> FNLPPGNYKKPKLLYCSNGGHFLRILPDGTVDGTRDRSDQHIQLQLSAESVGEVYIKSTETGQYLAMDTDGLLYGSQTPNEECLFLERLEENHYNTYISKKH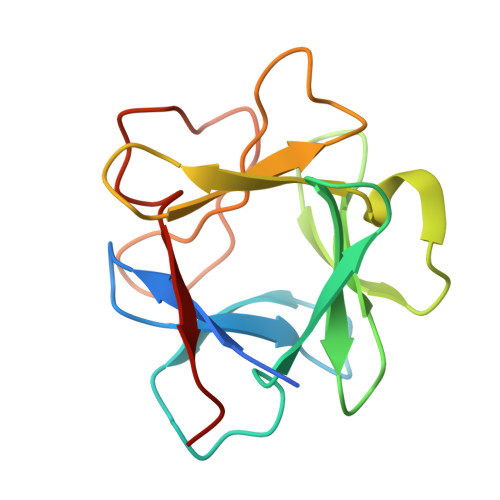AEKNWFVGLKKNGSCKRGPRTHYGQKAILFLPLPVSSD> KPCCDQCACTKSNPPQCRCSDMRLNSCHSACKSCICALSYPAQCFCVDITDFCYEPC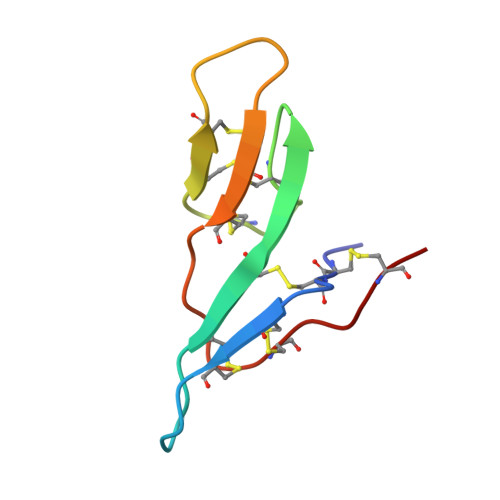K> MDQQSTRTDITVNVDGFWMLQALLDIRHVAPELRCRPYVSTDSNDWLNEHPGMAVMREQGIVVNDAVNEQVAAR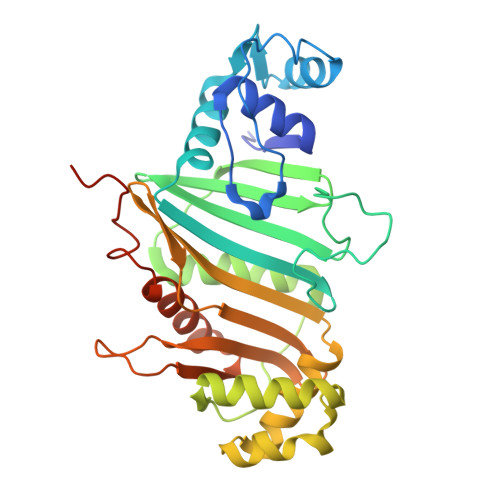MKVLAAPDLEVVALLSRGKLLYGVIDDENQPPGSRDIPDNEFRVVLARRGQHWVSAVRVGNDITVDDVTVSDSASIAALVMDGLESIHHADPAAINAVNVPMEEMLEATKSWQESGFNVFSGGDLRRMGISAATVAALGQALSDPAAEVAVYARQYRDDAKGPSASVLSLKDGSGGRIALYQQARTAGSGEAWLAICPATPQLVQVGVKTVLDTLPYGEWKTHSRVSSGGGSGGGSGGGS>[12x]MAKRRRKIKPMDDEQVLRHLDQLVNDALDFNSSELSKQRSEALKYYFGEPFGNERPGKSAIVSRDVQETVDWIMPSLMKVFTSGGQVVKYEPQTAEDVEQAEQETEYVNYLF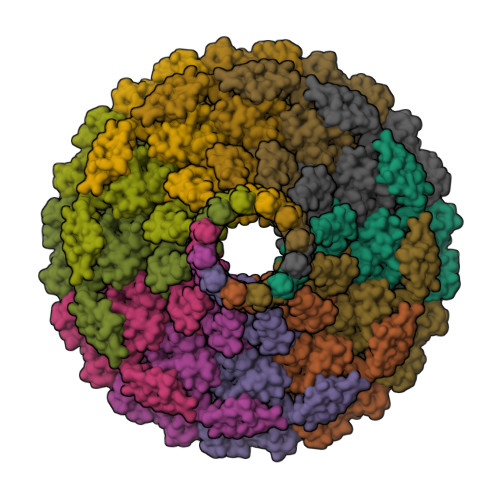MRKNEGFKVMFDWFQDTLMMKTGVVKVYVEEVLNPTFERFSGLSEEMVADILADPDTEILAQSVDEDGTYSIKIRKDKKKREIKVTCIKPENFLVDRLATCIDDARFLCHREKYTVSDLRLLGVPEDVLDELPYDEYEFSDSQPERLVRDNFDMTGQLQYNSGDDAEANREVWASECYTLLDVDGDGISELRRILYVGDYIISNEPWDCRPFADLNAYRIAHKFHGMSVYDKIRDIQEIRSVLMRNIMDNIYRTNQGRSVVLDGQVNLEDLLTNEAAGIVRVKAMNSIMPLETPQLSGEVYGMLDRLEADRGKRTGITDRTRGLDQNTLHSNQAAMSVNQLMTAAEQQIDLIARMFAETGVKRLFQLLHDHAIKYQNQEEVFQLRGKWVAINPANWRERSDLTVTVGIGNMNKDQQMLHLMRIWEMAQAVVGGGGLGVLVSEQNLYNILKEVTENAGYKDPDRFWTNPDSPEAQQAKAIREQKEAQPKPEDIKAQADAQRAQSDALAKQAEAQMKQVEAQIRLAEIELKKQEAVLQQREMALKEAELQLERDRFTWERARNEAEYHLEATQARAAYIGDGKVPETKKPSKAVRK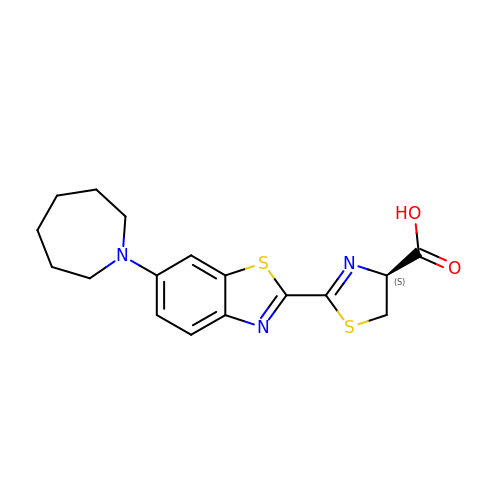(4S)-2-[6-(azepan-1-yl)-1,3-benzothiazol-2-yl]-4,5-dihydro-1,3-thiazole-4-carboxylic acid | C17 H19 N3 O2 S2 | GRFYBXURSQOJAN-CYBMUJFWSA-N>MPEPSISDLSFTSFVTNDDNLFEETFNFYTKLGFHATRSYVKDNRSDFELTGISTDSIKEIWLESFPLSEVVEASGGRELRKPLQESVGYESEALLGYSPYQSGGVVIKLRLSNHDLEKNNDLPGEVTFFTASIDKLKAKLIEIGAEIIPSKIDLVEFSTRDPMGDVISFSSYPSLNSKKITSPDFFLHPKKEVRSEESIVEQVKSEEGKKKIAIITSGGDAPGMNAAVRAVTRAGIFYGCKVYACYEGYTGLVKGGDMLKELQWQDVRGLLSIGGTIIGTARCKEFRERWGRLQACYNMVSNGIDALVVCGGDGSLTGADLFRKEWPELIKELLGEDKITKEQYETHRNLTIVGLVGSIDNDMCGTDSTIGAYSSLERIIELVDYIDATAASHSRAFVVEVMGRHCGWLGLMSGIATGADYIFIPERPPSESNWKDDLKKVCLRHREKGRRKTTVIVAEGAIDDQLNPITSEEVKDVLVEIGLDTRITRLGHVQRGGAPCAFDRFLATVQGVDAVRAVLESTPAIPSPVISILENKIVRQPLVESVAQTKTVSAAIEAKDFDKALQLRDQEFATSYENFLSVSKYDDGSYLVPESSRLNIAIIHVGAPTSALNPATRVATLNSLAKGHRVFAIRNGFAGLIRHGAVRELNWIDVEDWHNTGGSEIGTNRSLPSDDMGTVAYYFQQYKFDGLIIIGGFEAFTALYELDAARAQYPIFNIPMCCLPATVSNNVPGTEYSLGSDTCLNTLSGYCDAVKQSASASRRRTFVVEVQGGYSGYLASYAGLITGALAVYTPENPINLQTVQEDIELLTRTYEEDDGKNRSGKIFIHNEKASKVYTTDLIAAIIGEAGKGRFESRTAVPGHVQQGKSPSSIDRVNACRLAIKCCNFIEDANFQVKHNANLSADERHLRFFYDDGVKTSAVSGKSSVIDDNTSVVIGIQGSEVTFTPVKQLWENETHHKWRKGKNVHWEQLNIVSDLLSGRLSIRTT[4x];>[4x]MPDASLFNGTSFITLFAPNISLLQASIDFYTNFLGFAIRKNSNQKLFWLQLEEDQNNVSIQLILDPEHAASVSQIDQNIRNLTRSLYRKDWRSIQSNIAFKSSSLSKLVKLLKDGGHPVQQSPNEISPFEVYTVDPLGSLIGFSGFKNPFAVNERSLLPKVSEEKAYRAEDDSEKLLNPVRKTIGVMTSGGDSPGMNPFVRAVVRAGIYKGCKVFCIHEGYEGLVRGGEKYIKETQWHDVRGWLVEGGTNIGTARCKEFRERSGRLKACKNMIDMGIDALIVCGGDGSLTGADRFRSEWPSLIEELLQTEQISQQQFNTHQNLNICGAVGSIDNDMSSTDATIGAFSSLDRICRAIDYIDATANSHSRAFIVEVMGRHCGWLGLLAGLATSADYILIPEKPASSREWQDQMCDIVGKHRARGKRKTIVIVAEGAISNDLSPISCDQVKDVLVNRLGLDTRVTTLGHVQRGGTAVAFDRIYATLQGVEAVNAVLECDADTPSPMIAIKEDQITRVPLVDAVELTQQVAKSIESRNFKKAISLRDSEFVEHMKNFISTNSADHVPPSLPLEKRKKIAIINVGAPAGGMNSAVYSMATYCMSRGHVPYAIHNGFSGLARHESVRSINWLDIEGWGSLGGSEIGTNRTLPNDADIGMIAYFFEKYGFDGLILVGGFEAFISLHQLERARINYPSLRIPLVLIPATISNNVPGTEYSLGSDTCLNSFMEYCDVIKQSAAATRNRVFVVEVQGGNSGYIATHAQLACGAQISYVPEEGISLAQLEMDINSLKESFANDQGKTKSGRLILKSENASKVLTTEVISTIIDDEASGRFDSKTAIPGHVQQGGIPSPMDRVRASRFAIRAVSFIERHSDRCQTFKNSISFRQTDEITSTAVVLGIHKSQLRFTPIRQLYDFESDVPRRMRKNIFWSNVREISDMLSGRTSL;>MVTKDSIIRDLERENVGPEFGEFLNTLQTDLNSEKPPIEQVKSQLETHFNLAHETQEFSRKNDNAPVDKLLTNYYNNYEVNVLEFVLQMGFSRDLSIPLNVWFVLDMISQLSTSKQDLPLDYYLVLNNSQTGKYSDFVRYLIYEAVGAEIHCFEQGSMPEQYRSSRWEDKVKGPALANRGPIRGNVGAGDRKITFHLLCKKTARMILVGDDRETDFEMSDRSFVTLLLDYYQRVGTTKKIDLLLLTNNFDTNMNNKLQQLKILESLNMLKSNCYVLDYQITVDQVTANFNSYVEGI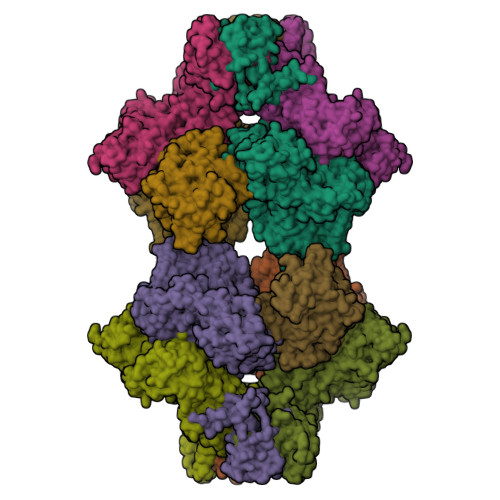PAFRRHEIANFLKKRKTPKNADELIFKYVGRWNICYQKKFHQGNISIHQISGYLD[4x]> AVPE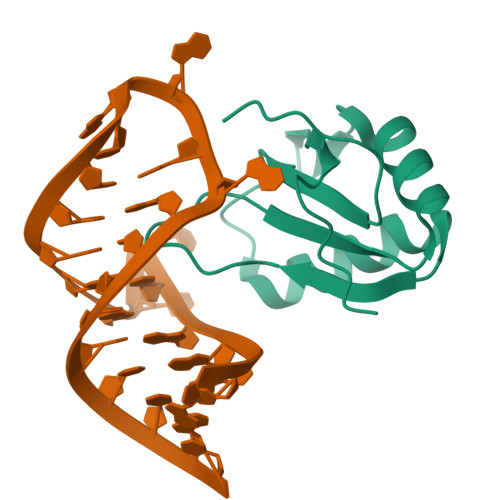TRPNHTIYINNLNSKIKKDELKKSLHAIFSRFGQILDILVPRTRTPRGQAFVIFKEVSSATNALRSMQGFPFYDKPMAIQYAKTDKRIP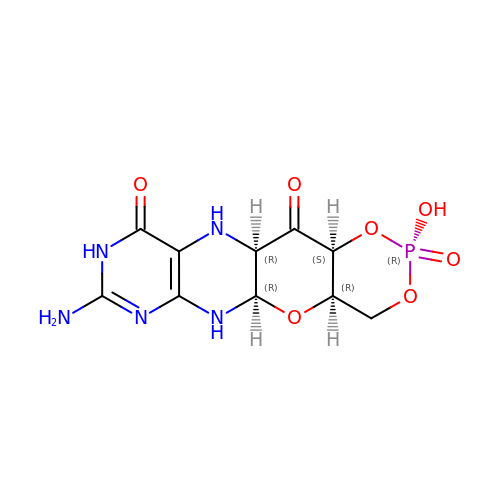(2R,4AR,5AR,11AR,12AS)-8-AMINO-2-HYDROXY-4A,5A,9,11,11A,12A-HEXAHYDRO[1,3,2]DIOXAPHOSPHININO[4',5':5,6]PYRANO[3,2-G]PTERIDINE-10,12(4H,6H)-DIONE 2-OXIDE | C10 H12 N5 O7 P | PWFXLXMPGSLEOZ-RNCCKPSGSA-N~{N}-[(2~{S},5~{S},14~{S})-2-[(4-fluorophenyl)methyl]-5-(hydroxymethyl)-9-methyl-3,8,15-tris(oxidanylidene)-1,4,9-triazacyclopentadec-14-yl]-5-methyl-1,2-oxazole-3-carboxamide | C26 H34 F N5 O6 | 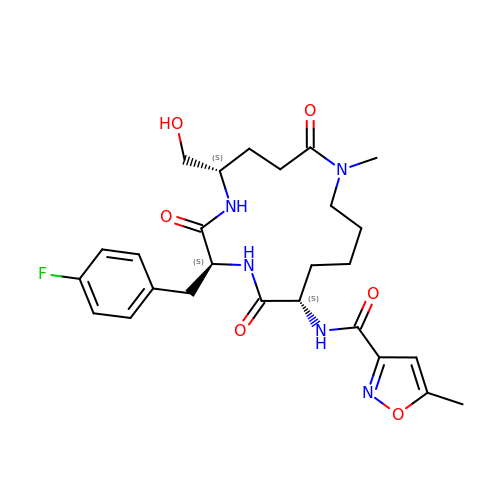NMKVYCKPYPCEGS-ACRUOGEOSA-N>SNAMGLDVRNNGNDNVEIRAAETRTAQRADEALETAADFAGQPKVTHTMRTINRTLSRRISRNTGSEQVLNLRRLMEKYLEDTRFKDDFIFVAVDPNQYSVPYPTLVVMSGAKVGDHNHFFGYVLPLVAGLAPLPRREEQGPHGNILVPRTWVDNLNGTFINEVMAAMYAAIGGKSNGTARIAGLAVVTNEITAESAHLATTLLSAADNAIQTAIEIRLGDKLGLPQFNLGMMASDQPISSVQYNTSGMQDSDIVGNPVRSDITVTISNRIRQAMSDYDSQQRLVATTGYIDLTYSPQNPTFNQGPVLVNGYPVP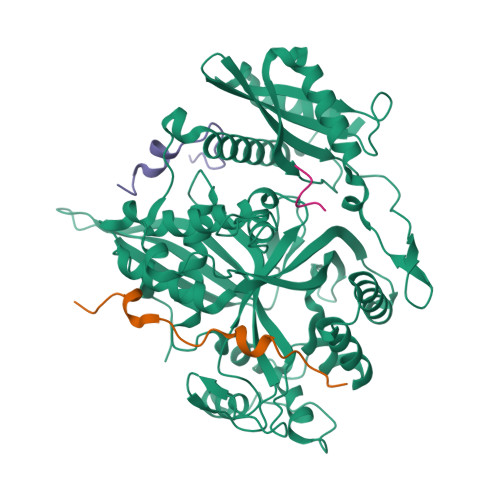PTVQYQPRYVMTSAYPLELDAFTPNTFVLGLIGTIATLNSGMAWAQSLISNAARGIGPHNPGALAMVLDPEVTAPLDLSTQTNEQIYKFLQQVLYPSLLISIDVPEEGEYSWLLRMIPAAEKIYTGKVEGEVREISEGYKALYRAFDDVTLGCFSKKYQYGLPLVYATGNRIPLGHYNHQDGHRHDIRDMDDLYMMNITNPDTVEAWEDSFDRTDMTMSQRVVARHEIIDRVLSGSWEQTGWAMRYDFDPLALQALIEAAADAGFTIRPENIQHLAGTAVRGNMAARARGLGNISGNIYARSDRPNVGVNNMGGAFNLF[4x]(2~{S},3~{R},4~{R},5~{S},6~{S})-2-(hydroxymethyl)-6-[(1~{S},2~{R},3~{R},4~{R},5'~{S},6~{S},7~{R},8~{S},9~{R},12~{R},13~{R},15~{S},16~{S},18~{R})-5',7,9,13-tetramethyl-3,15-bis(oxidanyl)spiro[5-oxapentacyclo[10.8.0.0^{2,9}.0^{4,8}.0^{13,18}]icosane-6,2'-oxane]-16-yl]oxy-oxane-3,4,5-triol 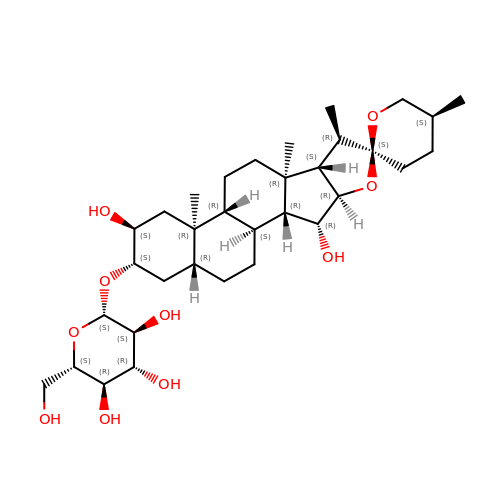| C33 H54 O10 | PDUIOILJOMOEIH-KWMFFDLQSA-N> NNEIMPGKMKVKATKG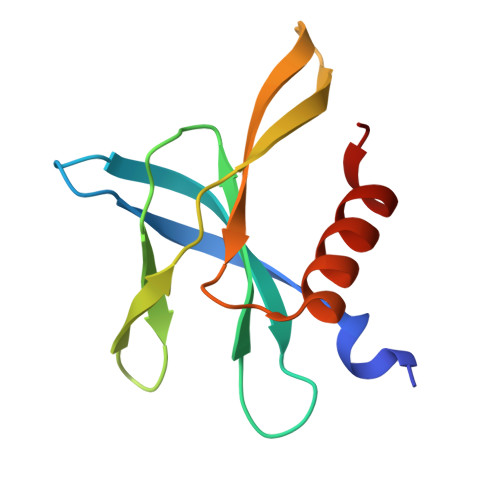EGDGGITSEGNALYNNEGGRAFMYAYVTTKPGMKYVKWEHDSGVVTVELEPPARFVIDTPTGPQIKYLYFVKNLNNLRRGAVLGYIGATVRLQ>[2x]MTKKIHINAFEMNCVGHIAHGLWRHPENQRHRYTDLNYWTELAQLLEKGKFDALFLADVVGIYDVYRQSRDTAVREAVQIPVNDPLMLISAMAYVTKHLAFAVTFSTTYEHPYGHARRMSTLDHLTKGRIAWNVVTSHLPSADKNFGIKKILEHDERYDLADEYLEVCY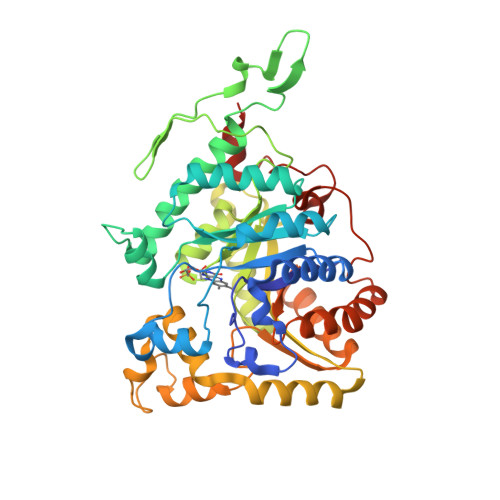KLWEGSWEDNAVIRDIENNIYTDPSKVHEINHSGKYFEVPGPHLCEPSPQRTPVIYQAGMSERGREFAAKHAECVFLGGKDVETLKFFVDDIRKRAKKYGRNPDHIKMFAGICVIVGKTHDEAMEKLNSFQKYWSLEGHLAHYGGGTGYDLSKYSSNDYIGSISVGEIINNMSKLDGKWFKLSVGTPKKVADEMQYLVEEAGIDGFNLVQYVSPGTFVDFIELVVPELQKRGLYRVDYEEGTYREKLFGKGNYRLPDDHIAARYRNISSNV>GPGSEFRQDKMREEGLQLVSMIREGEAAGACPEEIFSALQYSGTEVPLQWLRSELPYVLEMVAELAGQQDPGLGAFSCQEARRAWLDRHGNLDEAVEECVRTRRRKVQELQSLGFGPEEGSLQALFQHGGDVSRALTELQRQRLEPFRQRLWDSGPEPTPSWDGPD[2x];>[2x]DPAMQRCFSAAVYCAIS

To target disease-causing proteins that are inaccessible to small-molecule or antibody therapies, we are exploring the use of a nature-inspired drug modality that exploits the intrinsically favorable properties of synthetically constrained α-helical polypeptides (Helicons). Here, we report a rapid, high-throughput screening platform utilizing phage display that enables an unbiased mapping of the α-helical interactome of a given protein without any prior knowledge of its structure or known binding partners. Analysis of 14 high-resolution crystal structures of Helicon–protein complexes across six different protein domains reveals a range of binding modes, all of which are “side-on”, i.e., mediated exclusively by Helicon side-chains rather than involving main chain amide interactions. Biochemical and structural experiments demonstrate diverse functional impacts by the Helicons which bind these sites, including inhibition of protein–protein interactions, inhibition of enzymatic activity, induced conformational rearrangement, and induced dimerization.

We began with the E3 ubiquitin ligase RNF31, which is an integral component of the linear ubiquitin chain assembly complex. RNF31 is a 1,072-amino acid protein comprised of multiple folded and disordered regions. We screened two of the nonenzymatic folded domains, the PUB and UBA domains, each at multiple concentrations and in the presence or absence of a known binding partner. Binders to the RNF31 UBA domain, all of which compete with its partner Sharpin/SIPL1 in the phage screen, could also be grouped into at least two families. One of these families, comprised of Cluster C46 and C47, was characterized by a shared compact pharmacophore containing conserved leucine/phenylalanine, serine, valine, and tyrosine residues that was observed in two shifted registers. Biochemical characterization of members from C46 revealed that several Helicons bound with mid-nanomolar affinity. However, when we analyzed a cocrystal structure of one of these Helicons, FP06655, in complex with the RNF31 UBA domain, we observed an unexpectedly large conformational rearrangement when compared with the cocrystal structure of the RNF31 UBA domain in complex with its natural binding partner Sharpin/SIPL1. This rearrangement involves a significant rotation of the bundle of three N-terminal α-helices of the RNF31 UBA domain to form a groove in which the conserved leucine/phenylalanine and valine residues of FP06655 engage one wall of the groove, and the conserved serine and tyrosine residues engage the opposite wall, thereby stabilizing the RNF31 UBA domain in this induced fit. To confirm that this binding mode was not an artifact of crystallization, we showed that Sharpin UBL indeed competes with 5FAM-labeled FP06655 in solution. Together, these data illustrate the ability of Helicon binding to cause extreme induced fits, another feature of Helicon–protein recognition that we have now observed in several contexts.>MEHHHHHHTMLVYTEEDNISQLWGLYEMSREKLENDDIDASVSLVFGTIHEADRILRNTEDISTLPKDFHAAYSSALLAVSELFEIAQKRLKETNTEESYIDAAIERAQLGLDAPGNESRLFLALARAYLEKVRVLVWRHDNEESLANIPVTQLVNPYIEKAIQYLRPLAQDSTEYFDALTPDSLRPLYILSSYLFQFGDQFSEAFLLDVCSIITALWLKSVVDPNTPAYYKLIAQEA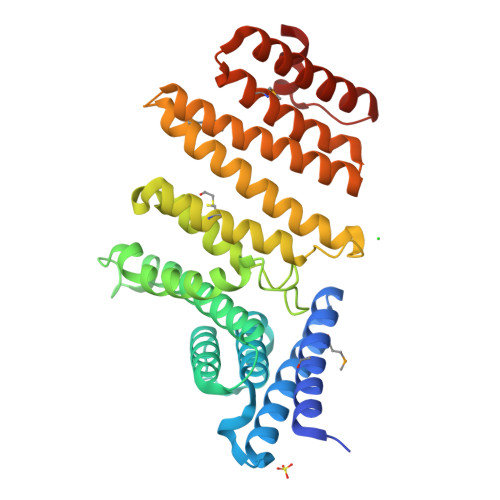VLNNYTTFAEYYMDLLDNSESNVDDLINKASSWLNNSVDTWNVIYTLDKSPERLLKLADIKMDLAQIVQDEASQDNYLKEACNAIKEAQGSGVELSPDYVEFVEAYSA[2x]>[8x]SNAMTRVAINGFGRIGRMVFRQAIKESAFEIVAINASYPSETLAHLIKYDTVHGKFDGTVEAFEDHLLVDGKMI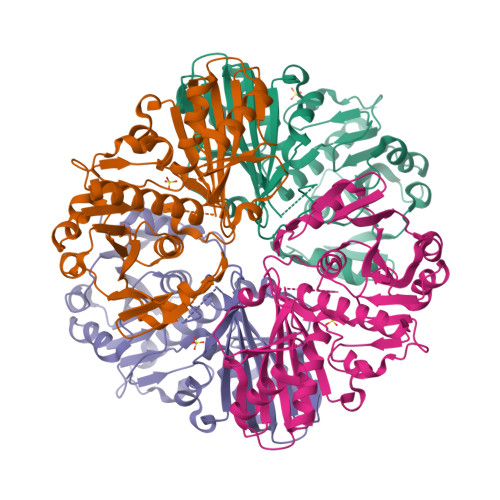RLLNNRDPKELPWTDLGVEVVIEATGKFNSKEKAILHVEAGAKKVILTAPGKNEDVTIVVGVNEDQLDITKHTVISNASCTTNCLAPVVKVLDEQFGIENGLMTTVHAYTNDQKNIDNPHKDLRRARACGQSIIPTTTGAAKALAKVLPHLNGKLHGMALRVPTPNVSLVDLVVDVKRDVTVEAINDAFKTVANGALKGIVEFSEEPLVSIDFNTNTHSAIIDGLSTMVMGDRKVKVLAWYDNEWGYSRRVVDLVTLVVDELAKQENVQHI BK polyomavirus (BKV) is an opportunistic pathogen that causes severe diseases in the immunosuppressed (Bennett et al., 2012). As expected, the BKV capsid has a T = 7d quasi-symmetry, and is built from 72 pentons of the major capsid protein VP1. Each of the six distinct conformations of VP1 present within the asymmetric unit of the capsid shares a common core fold (Figures 2B/2C), which is the β sandwich, “jelly roll” fold, characteristic of many viral capsid proteins. Crystal structures revealed that polyomavirus capsids consist of 360 copies of the major capsid protein VP1, which form 72 “pentons,” each consisting of a ring of five β barrel-containing VP1 monomers (Nilsson et al., 2005). Together, these form a T = 7d lattice, with a C-terminal arm from each VP1 making interactions with neighboring pentons to stabilize the capsid shell.

We present the 3.4-Å cryoelectron microscopy structure of native, infectious BKV in complex with the receptor fragment of GT1b ganglioside. Owing to the low concentration of our virus samples and low affinity of polyomavirus:receptor interactions (∼1–5 mM) (Neu et al., 2008, Stehle and Harrison, 1996), to study the BKV:GT1b structure we implemented an on-grid soaking protocol, where a 20 mM solution of the oligosaccharide portion of GT1b was applied to the carbon-immobilized virions for 30 s prior to blotting and plunge freezing. GT1b is a branched oligosaccharide, described previously as having “left” and “right” arms (Neu et al., 2013a). The disialic acid motif located on the right arm, of GT1b is well resolved in the 3.4 Å map. The binding mode is similar to that seen previously in a structure of GD3, an oligosaccharide that lacks a left arm, bound to a BKV VP1 penton. The left arm of GT1b is poorly resolved in our structure, indicating that it is not ordered at high resolution. To examine the possible location of the GT1b left arm, we emphasized lower-resolution features in the map by applying a 5 Å low-pass filter to the 3.4 Å map. This revealed bridges of density between Asp59 and Lys83 of VP1 and the GT1b density, consistent with previous mutagenesis data of these residues (D59Y and K83A), which resulted in significantly reduced BKV spread in cell culture (Neu et al., 2013a). MD simulations show that the left arm of GT1b is dynamic, explaining the lack of high-resolution density in our EM map, and its previous intractability to crystallographic studies. Low-resolution EM density and MD suggest a likely mechanism of binding for the left arm of GT1b, in which multiple, weak interactions occur with the VP1 surface.

>[6x]APTKRKGECPGAAPKKPKEPVQVPKLLIKGGVEVLEVKTGVDAITEVECFLNPEMGDPDENLRGFSLKLSAENDFSSDSPERKMLPCYSTARIPLPNLNEDLTCGNLLMWEAVTVQTEVIGITSMLNLHAGSQKVHEHGGGKPIQGSNFHFFAVGGDPLEMQGVLMNYRTKYPDGTITPKNPTAQSQVMNTDHKAYLDKNNAYPVECWVPDPSRNENTRYFGTFTGGENVPPVLHVTNTATTVLLDEQGVGPLCKADSLYVSAADICGLFTNSSGTQQWRGLARYFKIRLRKRSVKNPYPISFLLSDLINRRTQRVDGQPMYGMESQVEEVRVFDGTERLPGDPDMIRYIDKQGQLQTKML;> GAALALLGDLVASVSEAAAATGFSVAEIAAGEAAAAIEVQIASLATVEGITSTSEAIAAIGLTPQTYAVIAGAPGAIAGFAALIQTVSGISSLAQVGYRFFSDWDHKVSTVGLYQQSGMALELFNPDEYYDILFPGVNTFVNNIQYLDPRHWGPSLFATISQALWHVIRDDIPSITSQELQRRTERFFRDSLARFLEETTWTIVNAPINFYNYIQQYYSDLSPIRPSMVRQVAEREGTRVHFGHTYSIDDADSIEEVTQRMDLRNQQSVHSGEFIEKTIAPGGANQRTAPQWMLPLLLGLYGTVTPALEAYEDGPNQKKRRVSRGSSQKAKGTRASAKTTNKRRSRSSRS> GGSMGKTADNHGPVRSETAREGRENQVYSPVTGARLVAGCICLTPDKKQVLMITSSAHKKRWIVPAGGVEKDEPNYETTAQRETWEEAGCIGKIVAN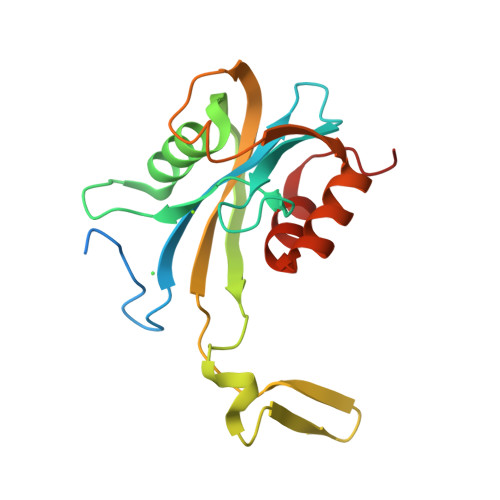LGTVEDMRPPKDWNKDIKQFENSRKDSEVAKHPPRTEFHFYELEIENLLDKFPECHKRHRKLYSYTEAKQNLIDAKRPELLEALNRSAIIKDDK The founding member of GH164, which we shall herein refer to as Bs164, originates from the enteric bacterium Bacteroides salyersiae CL02T12C01 and was initially reported by the authors to have α-mannosidase activity. In contrast to initial reports, this enzyme has no α-mannosidase activity; instead, Bs164 cleaves β-mannosidic linkages in aryl β-mannosidase and mannooligosaccharides. X-ray crystal structures of Bs164 reveal a homotrimeric quaternary structure with each individual chain containing three domains. The catalytic domain of Bs164 consists of a (β/α)8 barrel with catalytic residues on β-strands 4 and 7 placing this family in clan GH-A. NMR analysis revealed a retaining mechanism and site-directed mutagenesis confirmed the assignment of the nucleophile and acid/base catalytic residues.

To gain further insight into the mechanism and substrate recognition and confirm the assignment of the catalytic residues we produced structures of Bs164 in complex with 2,4-dinitrophenyl 2-deoxy-2-fluoro-mannoside (DNP-2FM), noeuromycin, and mannoimidazole through soaks of Bs164 crystals. Mannoimidazole and noeuromycin act as competitive inhibitors of Bs164 with inhibition constants (Ki) of 470 ± 60 μm and 340 ± 40 nm, respectively. The inhibition constant for noeuromycin is well in line with previous reports of β-mannosidase inhibition, however, inhibition by mannoimidazole notably is much worse than is seen for other β-mannosidases such as BtMan2A (Ki = 1.4 μm). The structure of the noeuromycin complex, in which a 1S5 conformation is observed, lends further support to this itinerary. The acid/base residue, Glu-160, is positioned to perform anti-protonation of the leaving group, typical of clan GH-A glycoside hydrolases. This residue forms hydrogen-bonding interactions with both the endocyclic nitrogen in noeuromycin and imidazole nitrogen in mannoimidazole, an interaction that is also seen in GH26 and GH113 β-mannanases and GH2 β-mannosidases. Another arginine, Arg-75 (which is bound to chlorine) hydrogen bonds to O3 of all inhibitors and the O2 of mannoimidazole and noeuromycin. The O2 hydroxyl also hydrogen bonds to Asn-159 in all three inhibitor structures and the nucleophile (Glu-297) in mannoimidazole and noeuromycin structures. The mannosidase inhibitors are recognized in the −1 subsite by eight polar amino acids, which are within hydrogen bonding distance to the substrate.

>[6x]MGSSHHHHHHSSGLEVLFQGPAERISKQSTPFVGAQIFIEPGQTQEQIEQWFKLLAESNMTTCRIRMFGKYMKTPSGTYDFTLFDRAFKLADKYHIKVYATLFPDTEFTDVGGFKFPHSREHQKEVEDYIKNVVSHFSQYKNLAAWVLINEPGTPNLPFNEPFTKERFSDWKKEHNFSEYNEKGYPVLNFEKENFIIDYHNWYLNWLANQVRLYDKQHDLHVNPHNVFKLSGLYDFPTWRTFLNSLGGSAHASWHFGYFPRKAYTVAMSANAELIRSGAGELPWLMTELQGGNNLYSGANPLCPTAEEIIQWLWINFATEAKGGIFWSFNARSTAAEAGEWAMINFKNKSSDRLIAAATIGKFITENVKMMSNIKTLNSGISILYNHESMWVEAAQTRGKLNGNGRSIGAVMCSPLSYFEALSETGLQANFKEIKEFDFSLNDYTDQVIILSHQIALDNKVIKQLESFVEKGGTLIADGLTGYYDYQAHSTVVSGFALENLFGSYPIEYKIKENLFSLDFEKDNYKLPAHLWKGTIETSKATPIMDKEGECIACINQYGKGKVFWIPSPIALGARESKDFSELSKLTVSLLPNKILNDNPHFDKHYKDVMMKSFKSNGTMYSLIINKSASVQTVDIVGGKGKAFILFANKNAHSTANKLTISPEETVIIKWKNN> MAGSGSERAEHQIILPESHLSSPLVKHKLLYYWKLTGLPLPDECDFDHLILSRQWKKILESSTPDIERMIKLGRSVHQTLSHSSKLTGILHPRCLEDLVGLDIPDSTNKFRRIEKKIQIHNTRYGEPFTRLCSYVEKKLLGSSWTHKIRRSEEFDSLRTDPAFWFHSSWSTAKFAWLHVKQIQRHLIVAARTRSASNKLVTLSHRSGQVFITPELVIVTHTNENKFTCLSQELVLMYADMMEGRDMVNIISSTAVHLRCLAEKIDDILRLVDALARDLGNQVYDVVALMEGFAYGAVQLLEPSGTFAGDFFSFNLQELRDTLICLLPQRIADSVTHAIANIFSGLEQNQAAEMLCLLRLWGHPLLESRAAAKAVRAQMCAPKMVDFDMILQVLSFFKGTIINGYRKKNAGVWPRVKAHTIYGNVIAQLHADSAEISHDIMLREYKNLSAIEFEACIEYDPVTNLSMFLKDKAIAHPRNNWLASFRRNLLSEEQKKNVQDSTSTNRLLIEFLESNDFDPYKEMEYLTTLEYLRDDSVAVSYSLKEEEVKVNGRIFAKLTKKLRNCQVMAEGILADQIAPFFQGNGVIQDSISLTKSMLAMSQLSYNSNRKRITDCKERVSSSRNHDLKGKHRRRVATFITTDLQKYCLNWRYQTIKLFAHAINQLMGLPHFFEWIHLRLMDTTMFVGDPFNPPSDPTDYDLTKVPNDDIYIVSARGGIEGLCQKLWTMISIAAIQLAAARSHCRVACMVQGDNQVIAVTREVRPDDSPESVLTQLHEASDNFFRELIHVNHLIGHNLKDRETIRSDTFFIYSKRIFKDGAILSQVLKNSSKLVLVSGDLSENTVMSCANISSTVARLCENGLPKDFCYYLNYLMSCIQTYFDSEFSITSSTQSGSNQSWINDIPFIHSYVLTPAQLGGLSNLQYSRLYTRNIGDPGTTAFAEVKRLEAVGLLGPNIMTNILTRPPGNGDWASLCNDPYSFNFESVASPSIVLKKHTQRVLFETCSNPLLSGVHTEDNEAEEKALAEYLLNQEVIHPRVAHAIMEASSVGRRKQIQGLVDTTNTVIKIALSRKPLGIKRLARIINYSSMHAMLFRDDVFLSNRANHPLVSSDMCSLALADYARNRSWSPLTGGRKILGVSNPDTIELVEGEILSISGGCSKCDSGDEQFTWFHLPSNIELTDDTSKNPPMRVPYLGSKTQERRAASLAKIAHMSPHVKAALRASSVLIWAYGDNDINWTAALKLARSRCNISSEYLRLLSPLPTAGNLQHRLDDGITQMTFTPASLYRVSPYVHISNDSQRLFTEEGVKEGNVVYQQIMLLGLSLIESLFPMTVTKTYDEITLHLHSKFSCCIREAPVAVPFELTGVAPDLRVVASNKFMYDPNPVAEGDFARLDLAIFKSYELNLESYSTVELMNILSISSGKLIGQSVVSYDEETSIKNDAIIVYDNTRNWISEAQNSDVVRLFEYAALEVLLDCSYQLYYLRVRGLNNVVLYMSDLYKNMPGILLSNIAATISHPIIHSRLHTVGLISHDGSHQLADTDFIELSAKLLVSCTRRVVSGLYAGNKYDLLFPSVLDDNLNEKMLQLISRLCCLYTVLFATTREIPKIRGLPAEEKCAMLTEYLLSDAVRPLLSPEQVDSITSPSIVTFPANLYYMSRKSLNLIREREDRDSILALMFPQEPLFEFPLVQDIGARVKDQLTMKPAAFLHELDLSAPARYDAYTLEQARSDCALADMGEDQLVRYLFRGVGTASSSWYKASHLLSVPEIRCARHGNSLYLAEGSGAIMSLLELHIPHETIYYNTLFSNEMNPPQRHFGPTPTQFLNSVVYRNLQAEVPCKDGFVQEFRTLWRENTEESDLTSDKAVGYITSVVPYRSVSLLHCDIEIPPGSNQSLLDQLATNLSLIAMHSVREGGVVIVKILYSMGYYFHLLVNLFTPCSVKGYVLSNGYACRGDMECYVVFVMGYLGGPTFVNEVVRMAKTLIQRHGTLLAKSDETALMALFTSQKQRVDNILSSPLPRLAKLLRRNIDTALIEAGGQPVRPFCAESLVNTLSDITQTTQVIASHIDTVIRSVIYMEAEGDLADTVFLFTPYNLSIDGKKRTSLKQCTRQILEVTILGLGPEDLNRVGDIISLILRGTISLEDLIPLRTYLKMSTCPKYLKSVLGLTKLREMFSDGSMLYLTRAQQKFYMKTVGNAVKGYYNSSKNENLYFQG;>MATFTDAEIDELFETSGTVIDSIITAQGKPVETVGRSAIPQGKTKALSLAWEKHGNTNTPAAQESAGEQDQHGQNQASNSNRATPEEGPHSSQAQAATQPQEDANESQLKTGASSSLLSMLDKLSNKSSNAKKGPPQSPPQQALHSKGSPAVEQTQHGANQGRAQQETGHQAAPSPGPPGTGVNIAFPGQRGVSPQSVGATQPAPQSGQNQGSTPASADHVQPPVDFVQAMMSMMEAISQRVSKIDYQLDLVLKQTSSIPTMRSEIQQLKTSVAVMEANLGMMKILDPGCANVSSLSDLRAVAKSHPVLIAGPGDPSPYVTQGGEIALNKLSQPVPHPSDLIKHATSGGPDIGIERDTVRALILSRPMHPSSSSKLLSKLDSAGSVEEIRKIKRLALNG[4x]

NDV RNA genome is replicated and transcribed by a multifunctional 250 kDa RNA-dependent RNA polymerase (L protein). The L protein consists of the N-terminal RNA-dependent RNA polymerase domain (RdRp), polyribonucleotidyl transferase domain (PRNTase), the connector domain (CD), the methyltransferase domain (MT), and C-terminal domain (CTD). The P protein adopts a unique tetrameric organization and interacts with L protein.

After motion correction, CTF estimation, 2D classification, 3D classification and 3D refinement, we obtained L-P complexes in three integrity states: the full-length L-P complex (Lf-P), core L-P complex (Lc-P) and core L-extended P complex (Lc-Pe). The final resolution of Lf-P complex, the Lc-P complex and Lc-Pe were 3.41 Å, 3.0 Å and 3.25 Å respectively. We also solved an Lc-Pe complex from which we built an extended region of the P-OD tetramer. Within the structure of this complex, we identified the OD (259-302) and XD (302-399) regions of the P proteins. We then modeled these regions in the cryo-EM density map to obtain the structure of Lc-Pe. Analysis of the complex structures showed that P1&P2 (P-OD regions, 261–289) interact with L, while P3 (260–312) and P4 (274–283, 308–315) are bound to the helix of P1&P2. Based on these findings, we built a more intact four-helix bundle of P-OD into the model of Lc-Pe. The other built region of P proteins was of similar length to its corresponding region present in the Lc-P complex structure.>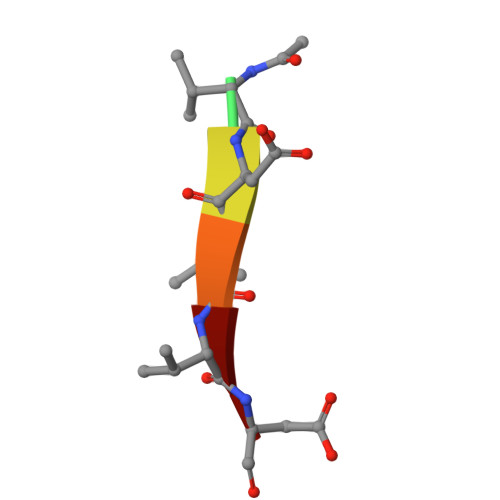 XVDVVD> MHQQHSKSENKPQQQRKKFEGPKREAILDLAKYKDSKIRVKLMGGKLVIGVLKGYDQLMNLVLDDTVEYMSNPDDENNTELISKNARKLGLTVIRG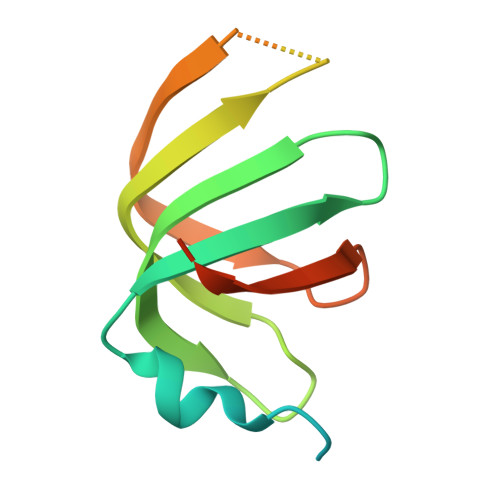TILVSLSSAEGSDVLYMQK>[4x]GPTRAELIDRFRRVAN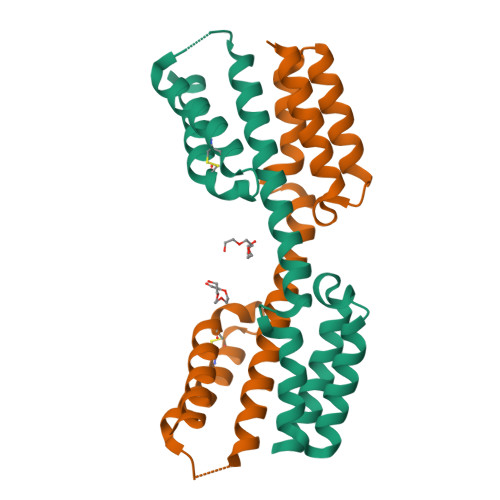EVRKASLLGSGDDVESILARTQAFLEEGDLDNAAREMNALTGWSKTLSRDWLAEVRKVLEVRQALEVIQAEARLQSLRLEGSGSRPLPESVEKARSEVVRCLREHDRRPLNCWQEVEAFKEEVRKLEKGWVDK>AEAGITGTWYNQLGSTFIVTAGADGALTGTYESAVGNAESRYVLTGRYDSAPATDGSGTALGWTVAWKNNYRNAHSATTWSGQYVGGAEARINTQWLLTSGTTEANA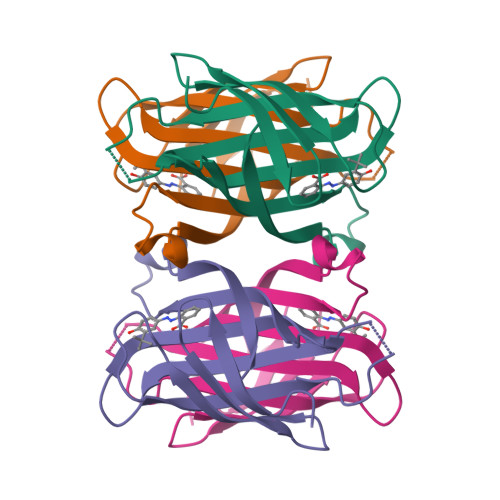WKSTLVGHDTFTKV[2x]> KNEEDESNDS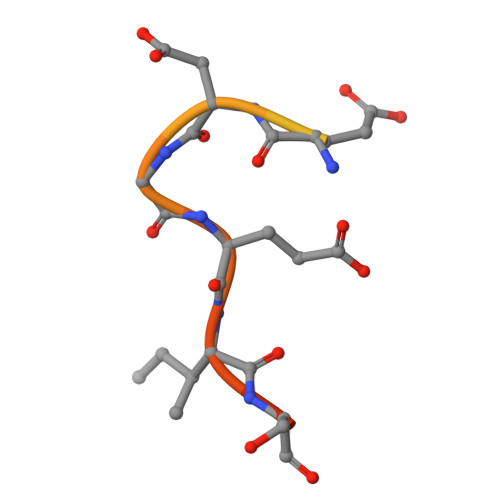DKEDGEISEDD> GLGQMLESMIDNTVRETVGAATSRDALPNTEASGPTHSKEIPALTAVETGATNPLVPSDTVQTRHVVQHRSRSESSIESFFARGACVTIMTVDNPASTTNKDKLFAVWKITYKDTVQLRRKLEFFTYSRFDMELTFVVTANFTETNNGHALNQVYQIMYVPPGAPVPEKWDDYTWQTSSNPSIFYTYGTAPARISVPYVGISNAYSHFYDGFSKVPLKDQSAALGDSLYGAASLN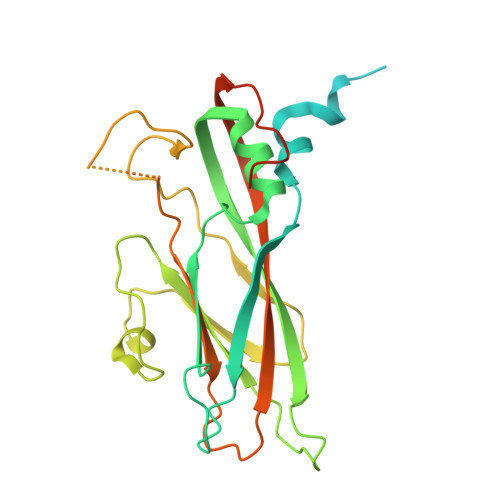DFGILAVRVVNDHNPTKVTSKIRVYLKPKHIRVWCPRPPRAVAYYGPGVDYKDGTLTPLSTKDLTTY> EKIAIRDFQVGDLVLIILDERHDNYVLFTVSPTLYFLHSESLPALDLKPGEGASGASR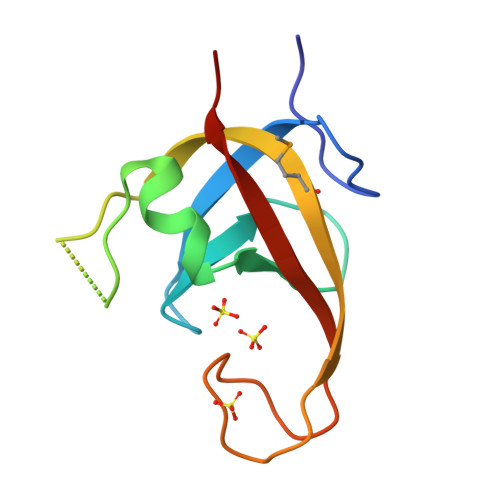RPWVLGKVMEKEYCQAKKAQNRFKVPLGTKFYRVKAVSWNKKV>GMVLTLSDLEKGYDKNLNQLSLSFLNLRDNDIPLLCEFLQNHPAITSLDLSHNDITANGVKLFVNKTSVSSLNISHNNIGPEGAQWLSEDNHITTLDVSFNEIGDEGVKALAANAKLITLYALYNKITKVGAGYLAQSNLKKIDLCFNSLEDEGVIALASNINIKELIASACDVSDIGAIELAKNNQLTLLILGKNAITDKSTLHFANNTSLSTLHLGSNQITAAGKKILETNTRITDLDLIGNPIEVHETDELNYSKKSPDSHSVFKFLQKFTFLSCMSPCQETAESDKGLNKKPN[8x];>[8x]GMAIAPQQIQERLKQEQYQKFVVADIGNFPHCLAQTPEGIASGQRYQKYSTNSLSRTPPFSQWGAPQLLTPKSAQEYIKFAQQRNKKSSFKIDGEAVRVSECSNFAYHSAGVLLDDPQIRTQYDVAVIGSMHSNGRYLHNITLLVPKGSRLPQPPQQLTAEVFPIGTLIVDPWAVGMGHPPEQALAIPKEQFAYNRSLFPATVNYQSALDESLTSTRTGQLTPYTGTPSRT

Among all bacterial pathogens, Legionella pneumophila maintains the largest known set of translocated substrates, delivering over 300 proteins to the host cell via its Type IVB, Icm/Dot translocation system. In at least nine instances, this regulation is direct—a hallmark of an emerging class of proteins called metaeffectors, or “effectors of effectors”. Through detailed structural and functional analysis, we show that metaeffector activity derives from a diverse range of mechanisms, shapes evolution, and can be used to reveal important aspects of each cognate effector's function. After release into the host cell, translocated bacterial substrates (effectors) regulate one another through several different functional interactions: indirectly, through counteracting modification of a shared host target, or directly through either steric complex formation or direct modification of one effector by another.

To that end, we performed detailed structure‐function analysis of a completely uncharacterized set of proteins: the putative metaeffector LegL1, a leucine‐rich repeat (LRR) protein (de Felipe et al, 2005), and its cognate effector, RavJ. After using Y2H and gel filtration analysis to demonstrate a physical interaction between LegL1 and the N‐terminal domain of RavJ, we cocrystallized and determined the crystal structure of this novel effector–effector complex (Table EV4). The co‐crystal complex of LegL1 (blue) bound to RavJ (1–226, red) was solved to a resolution of 2.0 Å. The heterocomplex has a 1:1 stoichiometry, with LegL1 forming a canonical LRR horseshoe‐shaped structure arching over and interacting with the RavJ active site identified above. LegL1 forms a canonical leucine‐rich repeat structure arching over the predicted active site of RavJ. The interface spans 1,240 Å2 and is reinforced by LegL1 K194 projecting into the RavJ active site where it forms a hydrogen bond with the predicted catalytic residue C101 (inset). LegL1 acts as a direct antagonist by blocking the active site of RavJ.>[2x]MKITVLVGGVGGARFLLGVQNLLGLGSFADGPSKHELTAVVNIGDDAWMHGVRICPDLDTCMYTLGGGIDPDRGWGHRNETWNAKEELAAYGVQPDWFGLGDRDLATHLVRSQMLRAGYPLSQVTEALCKRWQPGARLLP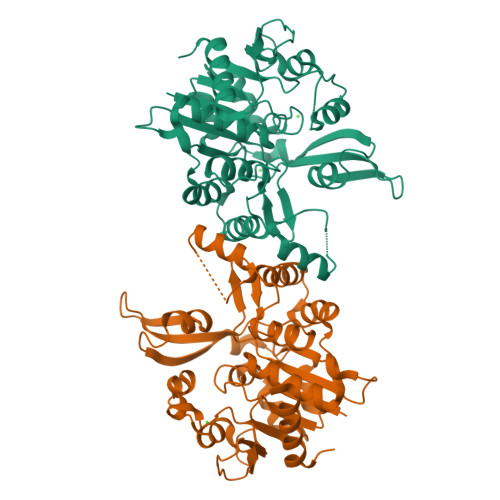ASDERSETHVVITDPTDGERRAIHFQEWWVRYRAKVPTHSFAYVGADQATAGPGVVEAIGDADIVLLAPSNPVVSIGPILQIPGIRGALRSTSAPVIGYSPIIAGKPLRGMADECLKVIGVESTSQAVGEFFGARAGTGLLDGWLVHEGDHAQIEGVKVKAVPLLMTDPEATAAMVRAGLDLAGVSL> MSELYQAKSETRSTITSSLKGIQPYKPTKATIWSRADALKVNEYDPTTTQPLVSGDFPVMSDEVFIWDTMPLRDIDGNIASVNGWSVIFTLTADRNPTAPEYQDEQGNYDITLDWNDRHGRAKMYFWYSRTGKDWIIGGRVMAEGVSPTAREWAGTPVLLNERGEIDLYYTAVTPGATVVKVRGRVVTTENGVEMVGFKKVKSLFEADGKMYQTESQNPYWAFRD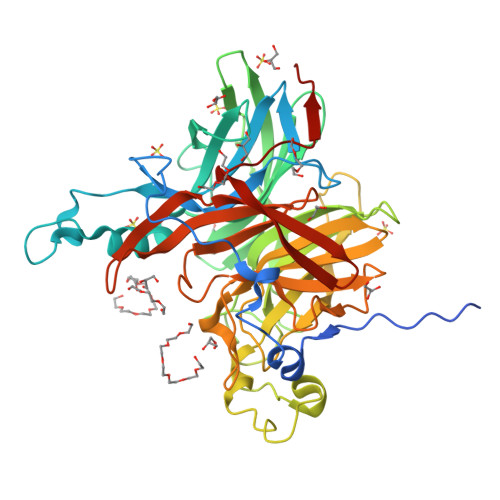PCPFRDPKSGKLYMLFEGNVAGERGSHVVGPDELGDVPPGYEDAGNSHFQTGCIGIAVCRDEDGDDWELLPPLITAVGVNDQTERPHFVFQDGKYYLFTISAKFTYGDGLTGPDGVYGFVSENLFGPYVPLNGSGLVLGNPPSQPYQTYSHYVMPNGLVTSFIDSVPTGEDSYRIGGTEAPTVLIKLKGAQTFVLEEFDYGYIPPMIDVKVEHHHHHH>[2x]MEFFGESWKKHLSGEFGKPYFIKLMGFVAEERKHYTVYPPPHQVFTWTQMCDIKDVKVVILGQDPYHGPNQAH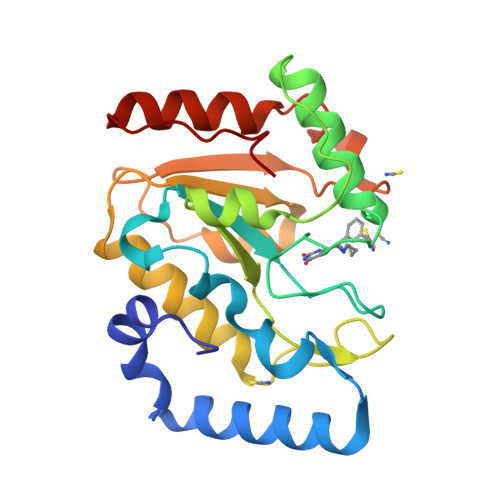GLCFSVQRPVPPPPSLENIYKELSTDIEDFVHPGHGDLSGWAKQGVLLLNAVLTVRAHQANSHKERGWEQFTDAVVSWLNQNSNGLVFLLWGSYAQKKGSAIDRKRHHVLQTAHPSPLSVYRGFFGCRHFSKTNELLQKSGKKPIDWKEL RIPK2 mediates inflammatory signaling by the bacteria‐sensing receptors NOD1 and NOD2. Here, we reveal that RIPK2 kinase activity is dispensable for NOD2 inflammatory signaling and show that RIPK2 inhibitors function instead by antagonizing XIAP‐binding and XIAP‐mediated ubiquitination of RIPK2. We map the XIAP binding site on RIPK2 to the loop between β2 and β3 of the N‐lobe of the kinase, which is in close proximity to the ATP‐binding pocket. Here, we reveal that RIPK2 kinase activity is dispensable for NOD2 inflammatory signaling, show that RIPK2 inhibitors function instead by antagonizing XIAP‐binding and XIAP‐mediated ubiquitination of RIPK2, and identify structural features of RIPK2 required for XIAP binding and for the design of efficient small molecule inhibitors of NOD1/2‐RIPK2‐dependent signaling.

To further understand the structural contributions of R1‐R3, we crystallized RIPK2 in complex with CSLP18, containing a hydrogen (H) in the R1 position compared to fluorine (F) and methoxy (OMe) in CSLP37 and 43, respectively (Table EV1). Overall, the complex with CSLP18 revealed RIPK2 in an inactive conformation previously shown for Type I1/2A inhibitors (Wu et al, 2015; Roskoski, 2016). Specifically, when compared to structures of active RIPK2 in complex with the ATP analog AMP‐PNP, the RIPK2‐CSLP18 structure showed mis‐orientation of the catalytic residues Asp146 of the HHD motif and Asp164 of the DFG motif, a slight misalignment of the R‐spine, a shifted P‐loop, and a completely disordered activation segment (AS) which is partially structured in active RIPK2 (Fig EV2D). The structure is refined at 3.2 Å resolution, and the electron density map is of sufficient quality in the region of the inhibitor to place the inhibitor and its relevant functional groups with reasonably good precision (Fig EV2E). CSLP18 forms two hydrogen bonds to the backbone of the hinge segment residues Glu96 and Met98, and the R3 sulfonamide forms a hydrogen bond to Asn151. The R3 hydrogen bond helps position the phenyl ring and R2 OMe group, which inserts into a sub‐pocket formed by the side chains of Glu66 and Leu70 of the αC‐helix. However, the R1 position does not optimally fill the hydrophobic pocket (termed deep pocket) formed by the side chains of Ala45, Lys47, Ile93, and gatekeeper Thr95 located on the β3 and β5 strands of the β sheet bundle. This is further revealed by the molecular docking of CSLP37 (R1 = F) and CSLP43 (R1 = OMe), which demonstrates that the larger R1 groups of these molecules more optimally fill the deep pocket (and EV2F). The RIPK2‐CSLP18 complex structure revealed the inhibitor occupying the ATP pocket of RIPK2 with the R1‐R3 groups of the inhibitor inserted into the deep pocket behind the adenine‐binding site. In sum, these data suggested that occupancy of the deep pocket is essential for the ability of CSLP analogs to bind endogenous RIPK2 and to block signaling by interfering with XIAP binding.

>SMGEAICSALPTIPYHKLADLRYLSRGASGTVSSARHADWRVQVAVKHLHIHTPLLDSERKDVLREAEILHKARFSYILPILGICNEPEFLGIVTEYMPNGSLNELLHRKTEYPDVAWPLRFRILHEIALGVNYLHNMTPPLLHHDLKTQNILLDNEFHVKIADFGLSKWRMMSLSQSRSSKSAPEGGTIIYMPPENYEPGQKSRASIKHDIYSYAVITWEVLSRKQPFEDVTNPLQIMYSVSQGHRPVINEESLPYDIPHRARMISLIESGWAQNPDERPSFLKCLIELEPVLRTFEEITFLEAVIQLKKTKLQSV[2x]4-amino-2-oxo-1,2-dihydropyrimidine-5-carboxylic 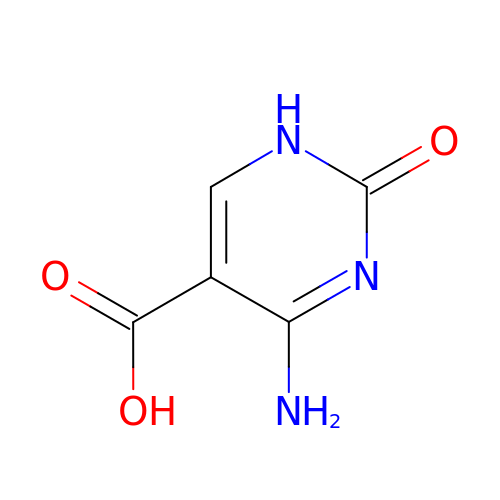acid | C5 H5 N3 O3 | BLQMCTXZEMGOJM-UHFFFAOYSA-N>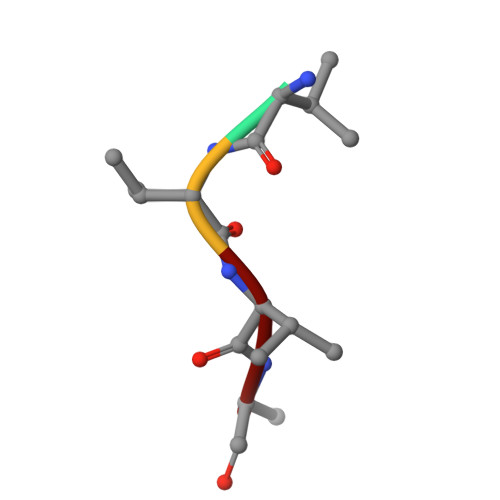 VVVA> MTKFKLLLAGSLVAIVSMGLLASNINEREKERVALNKTAHSQGIEGKAMSEEWARYYPRQFDSWKKTKESDNITDMLKEKPALVVAWAGYPFSKDYNAPRGHYYALQDNINTLRTGAPVDG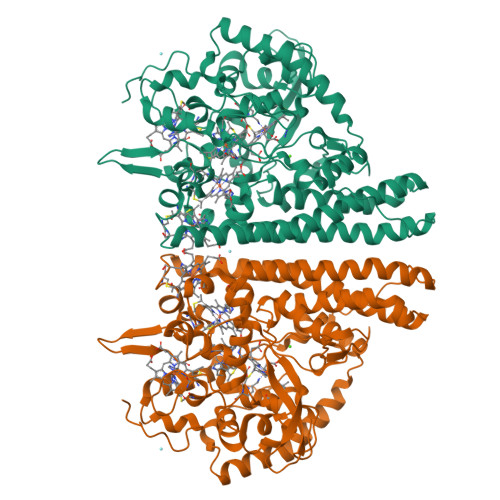KTGPLPSACWTCKSPDVPRIIEQDGELEYFTGKWAKYGDEIVNTIGCYNCHDDKSAELKSKVPYLDRGLSAAGFKTFAESTHQEKRSLVCAQCHVEYYFKKTEWKDDKGVDKTAMVVTLPWSKGISTEQMEAYYDEINFADWTHGISKTPMLKAQHPDWELYKTGIHGQKGVSCADCHMPYTQEGAVKYSDHKVGNPLDNMDKSCMNCHRESEQKLKDIVKQKFERKEFLQDIAFDNIGKAHLETGKAMELGATDAELKEIRTHIRHAQWRADMAIAGHGSFFHAPEEVLRLLASGNEEAQKARIKLVKVLAKYGAIDYVAPDFETKEKAQKLAKVDMEAFIAEKLKFKQTLEQEWKKQAIAKGRLNPESLKGVDEKSSYYDKTKK>PAFIVNTNVPRASVPDGFLSELTQQLAQATGKPPQYIAVHVVPDQLMAFGGSSEPCALCSLHSIGKIGGAQNRSYSKLLCGLLAERLRISPDRVYINY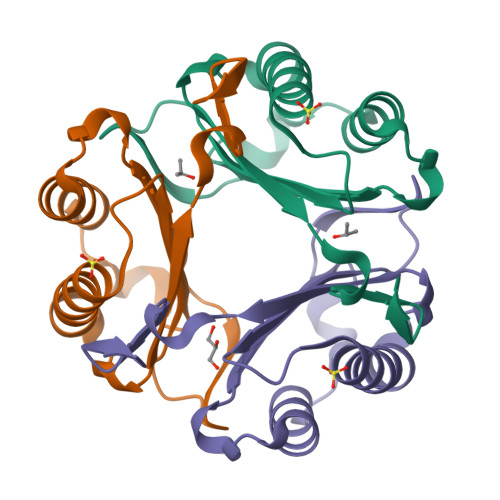YDMNAANVGWNNSTFA[3x]Here, we present InCellCryst, an advanced pipeline for producing homogeneous microcrystals directly within living insect cells. We have demonstrated the pipeline on five different proteins (IMPDH, HEX-1, Cathepsin B, Luciferase and EGFP-µNS), representing a selection of soluble proteins of different source organisms that crystallize in insect cells in their native compartment or, in case of peroxisomes, readily in the cytoplasm or nucleus of the cells. Importantly, as shown for IMPDH and HEX-1, InCellCryst can produce crystals from native protein sequences, without purification tags or even remnants of proteolytically removed tags, within a quasi-native cellular environment. The rich source of biomolecules in the cellular environment allows the identification of native ligands by co-crystallization at quasi physiological conditions, representing a unique feature of InCellCryst.

The 2nd generation cloning system (denoted as v2) uses cohesive ends produced by restriction enzymes KpnI and NheI for ligation, significantly improving the cloning efficiency, at the expense of two artificial residues at the N- and C-terminus of the target protein. The disruption of the native PTS1 signal by cloning into the pFB1 cyto and cyto v2 vectors transformed the hexagonal crystal blocks into a spindle-like shape. Whereas HEX-1 cyto and cyto v2 both formed spindle-like as well as bipyramidal crystals, HEX-1 ori crystals exhibit a hexagonal block shape. For HEX-1 ori and HEX-1 cyto crystals diffracted at 100 K one distinct unit cell population was found, whereas two unit cell populations were identified for HEX-1 cyto v2. For data collection from intact crystal-containing cells at 100 K, we carefully transferred the cells onto a MicroMesh mounted on a light microscope stage. Cells were then covered with 40 % PEG200 diluted in cell culture medium and manually frozen in liquid nitrogen. Serial diffraction datasets of the crystals contained in viable cells was performed using a helical grid scan approach, available at the EMBL P14 beamline located at the PETRA III storage ring (DESY, Hamburg, Germany). CrystFEL is optimized for still images in high multiplicity collected at RT at XFEL sources and thus, can be directly applied to serial synchrotron data. All HEX-1 structures show an increased flexibility between Phe145 and Ser151, the C-terminal loop region after the α-helix.

> MGTGYYDDDAHGHVEADAAPRATTGTGTGSASQTVTIPCHHIRLGDILILQGRPCQVIRISTSAATGQHRYLGVDLFTKQLHEESSFVSNPAPSVVVQTMLGPVFKQYRVLDMQDGSIVAMTETGDVKQNLPVIDQSSLWNRLQKAFESGRGSVRVLVVSDHGREMAVDMKVVHGSRLAS>MAHHHHHHMSEYLFTSESVSEGHPDKVADQVSDAILDAILAQDPKARVAAETLVNTGLCVLAGEITTTAQVDYIKVARETIKRIGYNSSELGFDANGCAVGVYYDQQSPDIAQGVNEGEGIDLNQGAGDQGLMFGYACDETPTLMPFAIYYSHRLMQRQSELRKDGRLPWLRPDAKAQLTVVYDSETGKVKRIDTVVLSTQHDPAISQEELSKAVIEQIIKPVLPPELLTDETKYLINPTGRFVIGGPQGDCGLTGRKIIVDTYGGAAPHGGGAFSGKDPSKV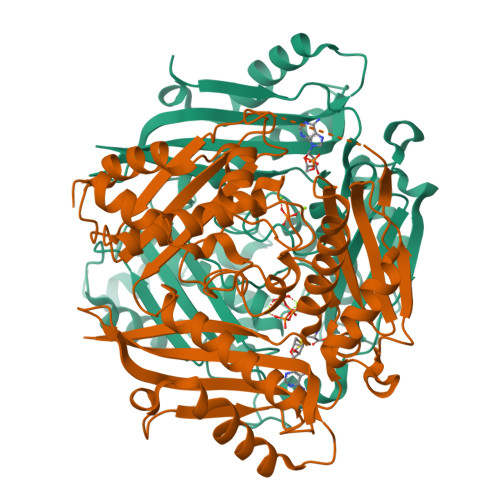DRSAAYACRYVAKNIVAAGLATQCQIQVSYAIGVAEPTSISIDTFGTGKISEEKLIALVCEHFDLRPKGIVQMLDLLRPIYGKSAAYGHFGREEPEFTWERTDKAASLKAAAGL[2x]>GPMQQANLGDGVATARLLSRSDWGARLPKSVEHFQGPAPYVIIHHSYMPAVCYSTPDCMKSMRDMQDFHQLERGWNDIGYSFGIGGDGMIYTGRGFNVIGAHAPKYNDKSVGIVLIGDWRTELPPKQMLDAAKNLIAFGVFKGYIDPAYKL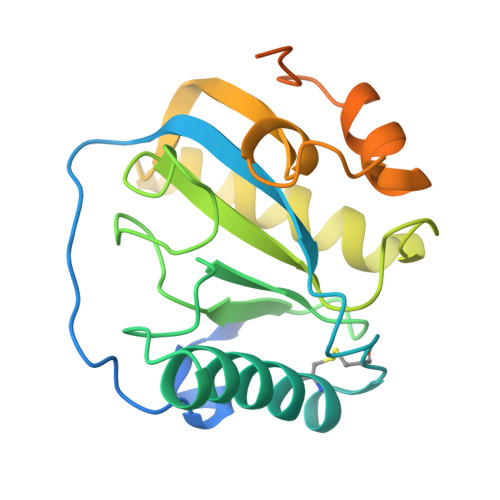LGHRQVRDTESPGGRLFAEISSWPHFTHINDTEGVSSTTAPVVPHVHPQAAAPQKPHQSPPAAPKV[2x]>[2x]MKELIKEHQKDINPALQLHDWVEYYRPFAANGQSANYIPALGKV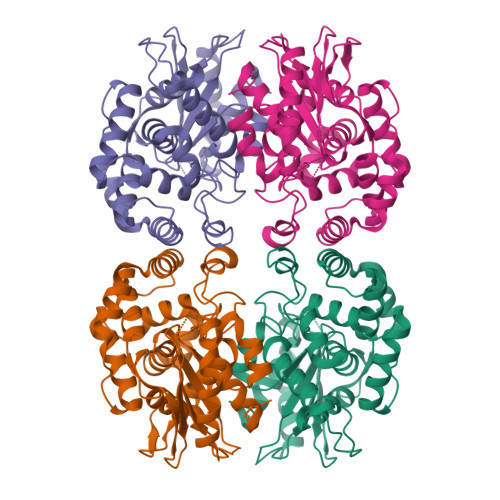NDSQLGICVLEPDGTMIHAGDWNVSFTMQSISKVISFIAACMSRGIPYVLDRVDVEPTGDAFNSIIRLEINKPGKPFNPMINAGALTIASILPGESAYEKLEFLYSVMETLIGKRPRIHEEVFRSEWETAHRNRALAYYLKETNFLEAEVEETLEVYLKQCAMESTTEDIALIGLILAHDGYHPIRHEQVIPKDVAKLAKALMLTCGMYNASGKYAAFVGVPAKSGVSGGIMALVPPSARREQPFQSGCGIGIYGPAIDEYGNSLTGGMLLKHMAQEWELSIF> MEALFPMSTDYSKMTDVNEIHDSAILEHFRNGIGHKTLVISPSYPYMFVGIIKELI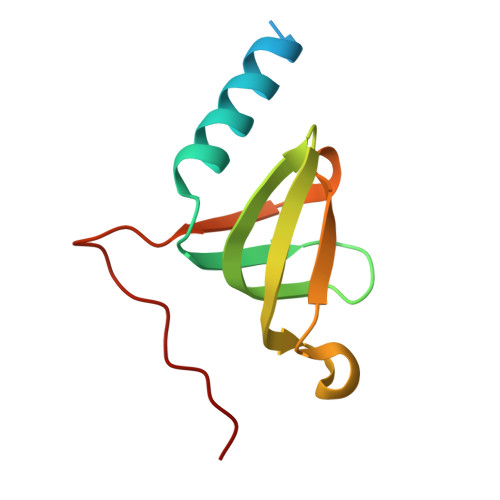GDTVMIDVETTHFAQLENREWYIHIHNIEVFYIERPGAPKIPKLEDY>[4x]LDATPLSSPRHVRIKNWGSGMTFQDTLHHKAKGILTCRSKSCLGSIMTPKSLTRGPRDKPTPPDELLPQAIEFVNQYYGSFKEAKIEEHLARVEAVTKEIETTGTYQLTGDELIFATKQAWRNAPRCIGRIQWSNLQVFDARSCSTAREMFEHICRHVRYSTNNGNIRSAITVFPQRSDGKHDFRVWNA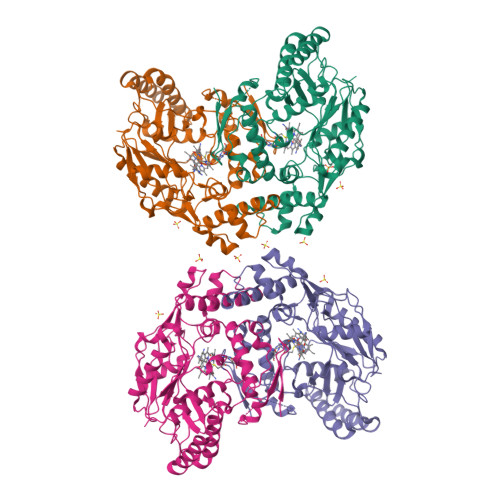QLIRYAGYQMPDGSIRGDPANVEFTQLCIDLGWKPKYGRFDVVPLVLQANGRDPELFEIPPDLVLEVAMEHPKYEWFRELELKWYALPAVANMLLEVGGLEFPGCPFNGWYMGTEIGVRDFCDVQRYNILEEVGRRMGLETHKLASLWKDQAVVEINIAVLHSFQKQNVTIMDHHSAAESFMKYMQNEYRSRGGCPADWIWLVPPMSGSITPVFHQEMLNYVLSPFYYYQVEAWKTHVWQDE>[2x]MSKEYHIDEEVGFALPNPQENLPDFYNDWMFIAKHLPDLIESGQLRERVEKLNMLSIDHLTDHKSQRLARL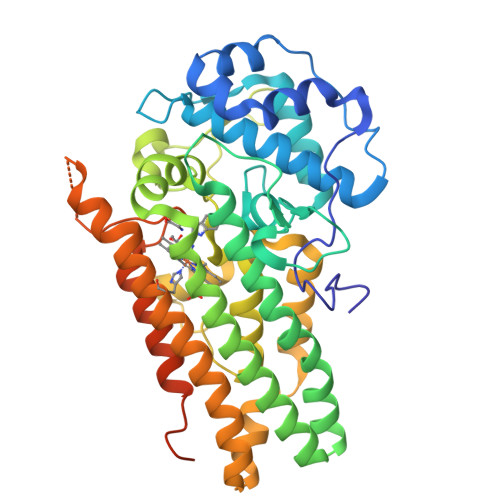VLGCITMAYVWGKGHGDVRKVLPRNIAVPYCQLSKKLELPPILVYADCVLANWKKKDPNKPLTYENMDVLFSFRDGDCSKGFFLVHLLVEIAAASAIKVIPTVFKAMQMQERDTLLKALLEIASCLEKALQVFHQIHDHVNPKAFFSVLRIYLSGWKGNPQLSDGLVYEGFWEDPKEFAGGSAGQSSVFQCFDVLLGIQQTAGGGHAAQFLQDMRRYMPPAHRNFLCSLESNPSVREFVLSKGDAGLREAYDACVKALVSLRSYHLQIVTKYILIPASQQPKENKTSEDPSKLEAKGTGGTDLMNFLKTVRSTTEKSLLKEGKGELNSKLEGKPIPNPLLGLDSTRTGHHHHHH>[6x]MTVAKAIFIKCGNLG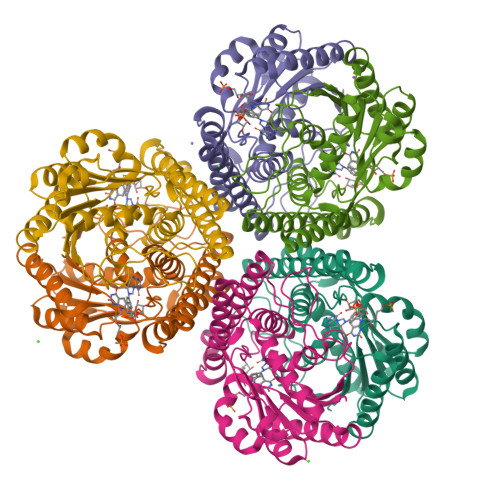TSMMMDMLLDERADREDVEFRVVGTSVKMDPECVEAAVEMALDIAEDFEPDFIVYGGPNPAAPGPSKAREMLADSEYPAVIIGDAPGLKVKDEMEEQGLGYILVKPDAMLGARREFLDPVEMAIYNADLMKVLAATGVFRVVQEAFDELIEKAKEDEISENDLPKLVIDRNTLLEREEFENPYAMVKAMAALEIAENVADVSVEGCFVEQDKERYVPIVASAHEMMRKAAELADEARELEKSNDAVLRTPHAPDGKVLSKRKFMEDPE[3-(benzyloxy)-4-methylphenyl]borinic acid | C14 H15 B O2 | 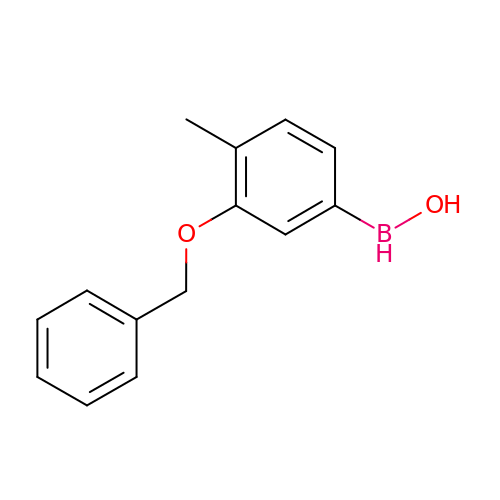AGVGVUFVBCPZKW-UHFFFAOYSA-N1,1,1-trifluoro-2-methylpropan-2-yl 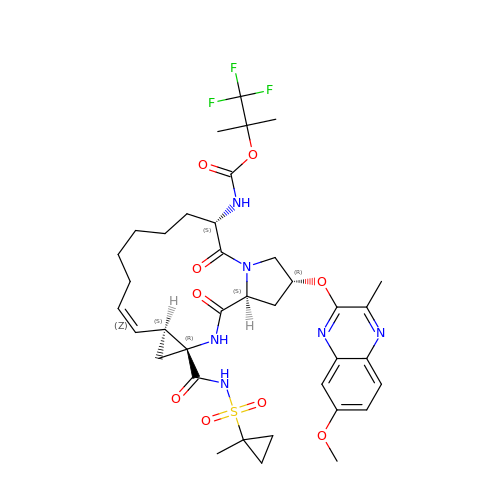[(2R,6S,12Z,13aS,14aR,16aS)-2-[(7-methoxy-3-methylquinoxalin-2-yl)oxy]-14a-{[(1-methylcyclopropyl)sulfonyl]carbamoyl}-5,16-dioxo-1,2,3,5,6,7,8,9,10,11,13a,14,14a,15,16,16a-hexadecahydrocyclopropa[e]pyrrolo[1,2-a][1,4]diazacyclopentadecin-6-yl]carbamate | C37 H47 F3 N6 O9 S | ZOQBCVXDXFPSSL-DDAYHPHASA-N>[2x]MLMVDEQLKIGATPMYSPSHNPIVIADDMEKGGSDSDSLPSSPTHHHELYRRPWIHEPRATNFFVRLITSLYALILTIISLVVEVSPTWRTDMWLAETIFYISMYGVGILFFAYCYIFIIYPGPYNQLISVLRKYKIIKNSEVWFIMQSQHNGEGAGTLYLRLGALFFGSVGIVLFGLELFLCIENVACKKVAIAKMIVAIVFTFIQMHFIFCNSKITVNSSRKIVAFGMMHLISVNLWTWFRFVLAKQEAKAHKKAQLKQTFRKYYSSSSSSSSEEIHELISAVLNSTLNNTPATKTMEPVASRLFALEHFGDVATFLTTCIVEYSLIGAAIMFILWKSIGQNNHQQSNSGKRKVKMRIDCSSSSTGLFAGIIFLIGSLVSMGMYTIFESLRNSSGAQLVFGIVDLSLFSIALGACIIGLWRMRHLQYRLHAHGEVIDEILLIIGLIGEILYCAVGIDVFITCRRSADLTVSALPAFVFVIRMIQVVVQAAFILTTSRLRCLSKYSMKYKPGKEIITFLLVSNVTLFVFHTFEGMKSSFGFSSKAATQYNYIIYAVGPLLVFYRFHSSACLAEIWKHTYSTKSNEYDHEHMSLSDSNLTAITPISDIKEIPSPQLLKH

The otopetrin (OTOP) proteins were recently characterized as extracellular proton-activated proton channels. Several recent OTOP channel structures demonstrated that the channels form a dimer with each subunit adopting a double-barrel architecture. In this study, we performed structural and functional characterization of the Caenorhabditis elegans OTOP8 (CeOTOP8) and mouse OTOP2 (mOTOP2) and illuminated a set of conformational changes related to the proton-conducting process in OTOP. Combining the structural information from both channels, we propose a working model describing the multi-step conformational changes during the proton conducting process.

The WT CeOTOP8 was overexpressed in HEK293F cells and purified in glyco-diosgenin (GDN) detergent. Its structures were determined at pH 5.0 and 8.0 using single-particle cryo-EM. At high pH, the CeOTOP8 inter-barrel interface adopts an intriguing structure. The Glu325 side chain points down towards the intracellular side whereas the His567 imidazole ring adopts two alternative conformations. The His567 side chain flips up toward the extracellular side in its major conformation, forming a salt bridge with Glu325. This structure likely represents a transient state in which the protonated Glu325 is transferring its proton to His567. In its minor conformation, the His567 side chain remains downward-facing in the cavity and exposed to the cytosolic solution. Firstly, TM12 of CeOTOP8 forms a bent helix at low pH with a kink at a highly conserved proline (Pro559) residue, whereas the N-terminal part of the TM12 helix before Pro559 unwinds to a loop at high pH. This helix-to-loop structural transition allows the Phe563 side chain to rotate upward, vacating the space necessary to accommodate the upward flip of the His567 imidazole as well as the downward rotation of Glu325 side chain. Thus, this structural transition appears to be prerequisite for the formation of the proton-transferring bridge between Glu325 and His567. The other structural change is that the residues 244–270 after the C-terminus of TM5 are disordered at low pH but form a helix that extends seamlessly after TM5 at high pH.>IVGGRRARPHAWPFMVSLQLRGGHFCGATLIAPNFVMSAAHCVANVNVRAVRVVLGAHNLSRREPTRQVFAVQRIFE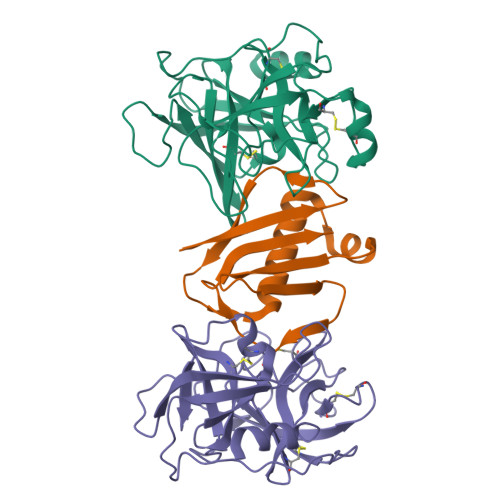NGYDPVNLLNDIVILQLNGSATINANVQVAQLPAQGRRLGNGVQCLAMGWGLLGRNRGIASVLQELNVTVVTSLCRRSNVCTLVRGRQAGVCFGDSGSPLVCNGLIHGIASFVRGGCASGLYPDAFAPVAQFVNWIDSIIQ[4x];>[4x]GSTVQVPYTITVNGTSQNILSNLTFNKNQNISYKDLEGKVKSVLESNRGITDVDLRLSKQAKYTVNFKNGTKKVIDLKSGIYTANLINSSDIKSININVD;>[4x]IIGGRESRPHSRPYMAYLQIQSPAGQSRCGGFLVREDFVLTAAHCWGSNINVTLGAHNIQRRENTQQHITARRAIRHPQYNQRTIQNDIMLLQLSRRVRRNRNVNPVALPRAQEGLRPGTLCTVAGWGRVSMRRGTDTLREVQLRVQRDRQCLRIFGSYDPRRQICVGDRRERKAAFKGDSGGPLLCNNVAHGIVSYGKSSGVPPEVFTRVSSFLPWIRTTMR> MAQPPRPAEEYDDDVQEDEDELKEGELDDDESHEAASEGGEAAAGDEEAEDDEQDEEDGDEDSQPWAGLNRLPERDDMLDILNELRAEGRKQLTVLLLGKSSVGKSSLINSLLGEAVVRVQAFKLQADTDITTTVVRQVAVGNSEVDGFRLKLIDTCGLEDPEAGDTVNLGALSKIAEDVRGVGIDVVLYCDRLDLYRVDPLDKAI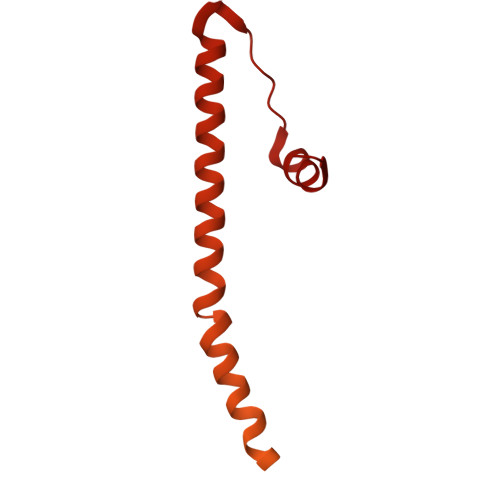IDAISSTFGRGIWRRTVVALTHANLVQTPPGTDYDSFVNGRVRLIRGAVRGPLFFRPSLPVALVENSETCPVSSESGFRVLPDGEPWLVALVSQLVDMAAARRRPYKYHPRLSSKPSHRFRWLLPVAIAAEVLFYRRFLHPRLDDNQRRVEREEERVWALRGQQRRALGLHRPHRPDKDAAWRLEQMYDDD[(2~{S})-2-(6-chloranyl-7-methyl-1~{H}-benzimidazol-2-yl)-2-methyl-pyrrolidin-1-yl]-[5-methoxy-2-(1,2,3-triazol-2-yl)phenyl]methanone 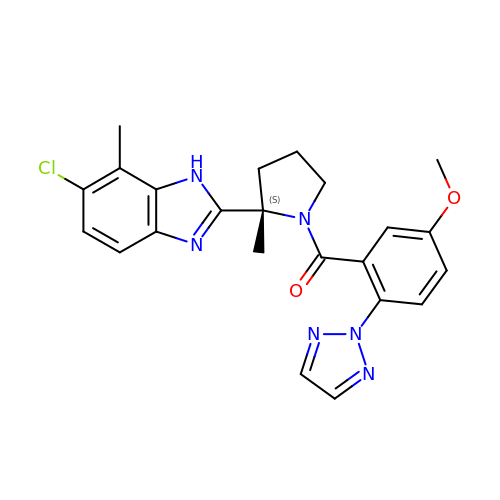| C23 H23 Cl N6 O2 | NBGABHGMJVIVBW-QHCPKHFHSA-N> GSHMANKAVNDFILAMNYDKKKLLTHQGESIENRFIKEGNQLPDEFVVIERKKRSLSTNTSDISVTATNDSRLYPGALLVVDETLLENNPTLLAVDRAPMTYSIDLPGLASSDSFLQVEDPSNSSVRGAVNDLLAKWHQDYGQVNNVPARMQYEKITAHSMEQLKVKFGSDFEKTGNSLDIDFNSVHSGEKQIQIVNFKQIYYTVSVDAVKNPGDVFQDTVTVEDLKQRGISAERPLVYISSVAYGRQVYLKLETTSKSDEVEAAFEALIKGVKVAPQTEWKQILDNTEVKAVILGGDPSSGARVVTGKVDMVEDLIQEGSRFTADHPGLPISYTTSFLRDNVVATFQNSTDYVETKVTAYRNGDLLLDHSGAYVAQYYITWDELSYDHQGKEVLTPKAWDRNGQDLTAHFTTSIPL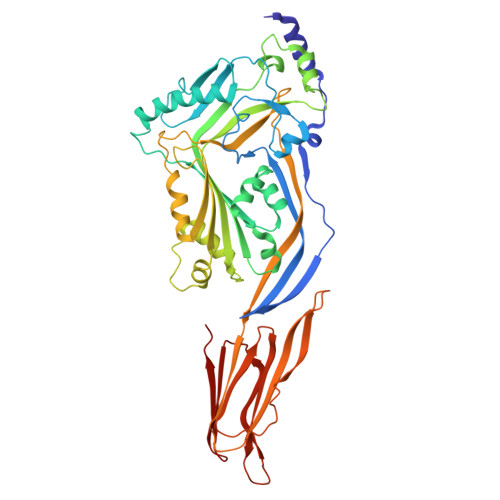KGNVRNLSVKIRECTGLAWEWWRTVYEKTDLPLVRKRTISIWGTTLYPQVEDKVEND>MHHHHHHAMEEVTIKANLIFANGSTQTAEFKGTFEKATSEAYAYADTLKKDNGEWTVDV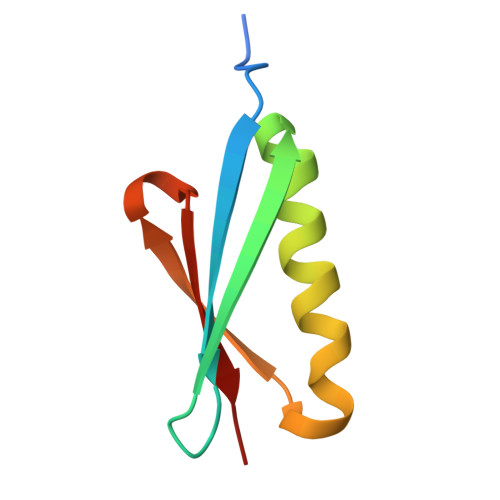ADKGYTLNIKFAG[3x]5-[(3aS,4S,6aR)-2-oxo-hexahydro-1H-thieno[3,4- 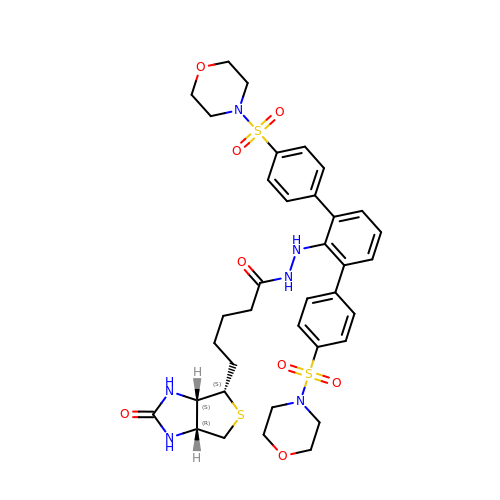d]imidazolidin-4-yl]-N'-{2,6-bis[4-(morpholine-4- sulfonyl)phenyl]phenyl}pentanehydrazide | C36 H44 N6 O8 S3 | VJIGZSIHTAESLS-QVXXBSHFSA-N> AQCEATVESNDAMQYNVKEIVVDKSCKQFTMHLKHVGKMAKVAMGHNLVLTKDADKQAVATDGMGAGLAQDYVKAGDTRVIAHTKVIGGGESDSVTFDVSKIAAGENYAYFCSFPGHWAMMKGTLK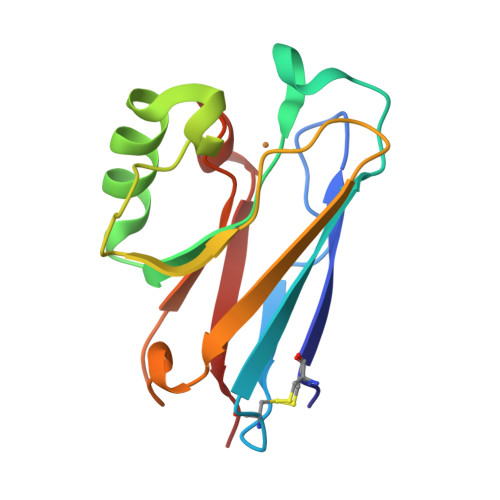LGS> GAVSETISETAWCLDGFERPTGVNPVIKPLPTKFYCPMREDSVAWEESDTFNPAATIYDGKIVVMYRAEDNSAQGIGSRTSRLGYATSTDGIHFERDTKPAFYPAKDNQAENECPGGTEDPRIAMTEDGTYVLLYTQWNRKVPRLAVATSKDLKHWTKFGPAFEKAYNGKFKDEATKSASLVTTLKGDKQVIAKVNGKYFMYWGEKNVYAATSDNLIDWDPLLDENGELLKLFSPRSGYFDSQLTECGPPAILTKDGIVLLYNGKNEPGEKGDTAYPANSYCAGQALFDVNNPTKLIGRLDKPFLQPTDDFEKS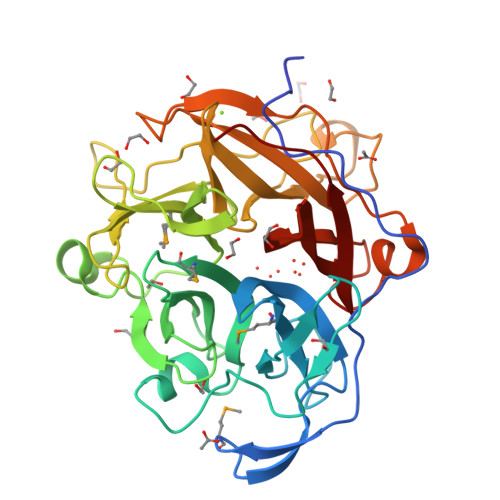GQYPAGTVFVEGLVYYRNKWYLYYGCADSFVAVAVSDKQLNF>MGHHHHHHENLYFQGHFVQQKVKVFRAADPLVGVFLWGVAHSINELSQVPPPVMLLPDDFKASSKIKVNNHLFHRENLPSHFKFKEYCPQVFRNLRDRFGIDDQDYLVSLTRNPPSESEGSDGRFLISYDRTLVIKEVSSEDIADMHSNLSNYHQYIVKCHGNTLLPQFLGMYRVSVDNEDSYMLVMRNMFSHRLPVHRKYDLKGSLVSREASDKEKVKELPTLKDMDFLNKNQKVYIGEEEKKIFLEKLKRDVEFLVQLKIMDYSLLLGIHDIIRGSEPEEELGPGEFESFIDVYAIRSAEGAPQKEVYFMGLIDILTQYDAKKKAAH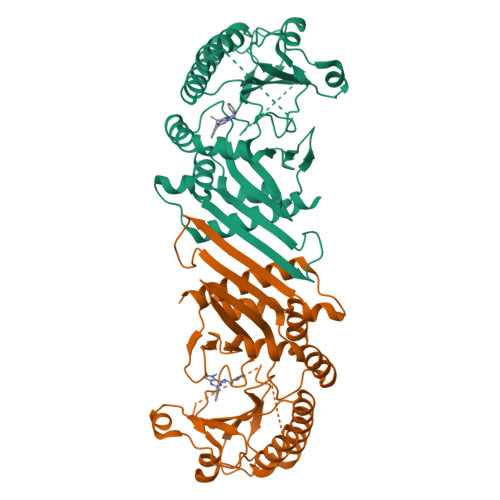AAKTVKHGAGAEISTVHPEQYAKRFLDFITNIFA[4x]> TDNIRPTYQTDANGTYPTNSWQVTGQQNVINQRGGDQVSGWDNNTIWNGDATDTTNSYLKFGDPNNPDYQIRKYAKETNTPGLYDVYLNVKGNKQQNVKPVDIVLVVDMSGSMESNRWGTNRAGAVRTGVKNFLTSIQNAGLGNYVNVGLIGFSSPGYIGGKSGYISVKLGKAGNASQQQAINGALSPRFQGGTYTQIGLRQGSAMLNADTSGNKKMMILLTDGVPTFSNEVINSEWINGTLYGTNFGSSRDEPGNTARLRWPYTDSSGHYIYDTWPATLGEAKIAKDSGNEVHALGIQLADDDHYMTKEKIRQNMQLITNSPDLYEDADSADAVEAYLNNQAKDIIKNFNTVTDGTITDPIGTQFQYANNQATVTSVGKQTVPASELPSAAIQDGQLTVNHMNLGQDQEVQIHYQVRIKTEDAGFKPDFWYQMNGETLLTPKAGAAAVDFGIPSGRAPATTVYVQKQWRQLSNQSLPDTLNVTVQRKVADGSLDPNWQQTLVLKKADNWKASFTAPAYNNQGQSFSYVVKSEDASGIDLSSFISSQNMDQQTATLTLTNQQYGFQFQKKTTDGTDLSADQ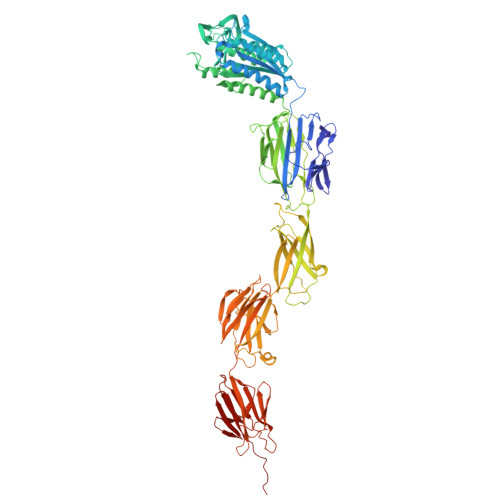LKAMQFNLTQYSDNSFQQASKTNAITSTDLQALAPGYYGIQEAAAPTGYQLDGTTYLFQLTSDGQWQYHGTKDNVTSGSVINGQQTLNPVGDKSDDFTVTGDHQQILTLTKYDEPKPSMTLRVIKQDNQSQYLAGAAFTLQPSAGEAETITSSATSEGQAFATKLVADGTYTMSETKAPDGYQSNPAKIAIQVATTGKEATVTIDGEALKPGESKNGYTLAIDGSTITLQAINQPLAILPL>NTKYNKEFLLYLA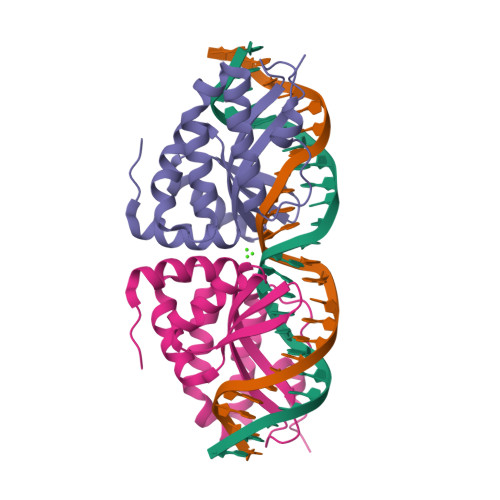GFVDGDGSIIAQIKPNQSYKFKHQLSLTFQVTQKTQRRWFLDKLVDEIGVGYVRDRGSVSDYILSEIKPLHNFLTQLQPFLKLKQKQANLVLKIIEQLPSAKESPDKFLEVCTWVDQIAALNDSKTRKTTSETVRAVLD[2x]> GPLGSWVIPPISCPENEKGEFPKNLVQIKSNRDKETKVFYSITGQGADKPPVGVFIIERETGWLKVTQPLDREAIAKYILYSH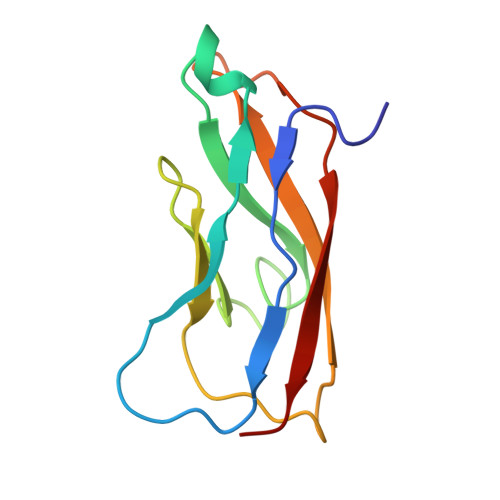AVSSNGNAVEDPMEIVITVTDA>[2x]XGEA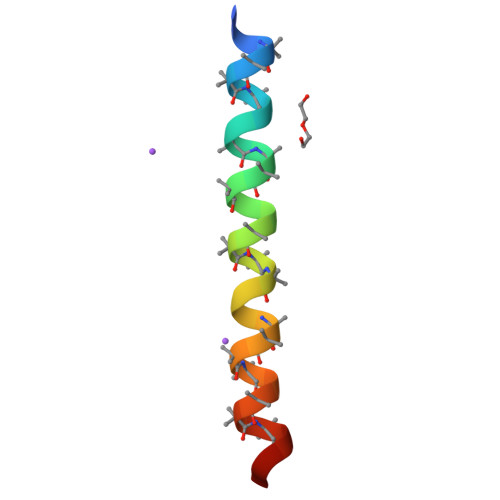AAAKEAAAAKEAAAAKEAAAAKAAAWKGX N-oxidanyl-4-[(4-sulfamoylphenyl)methyl]benzamide 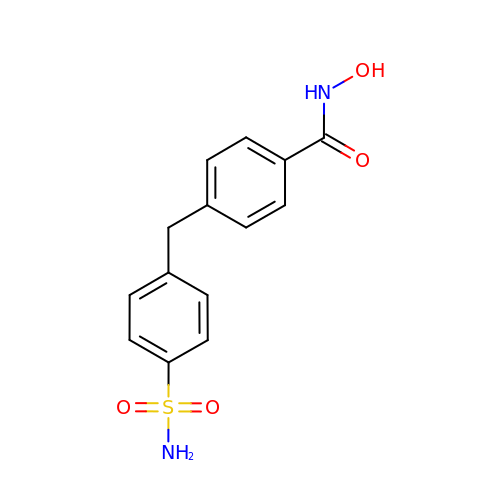| C14 H14 N2 O4 S | ZYVHYCNSGQRCBB-UHFFFAOYSA-N> APDGKKGEAGR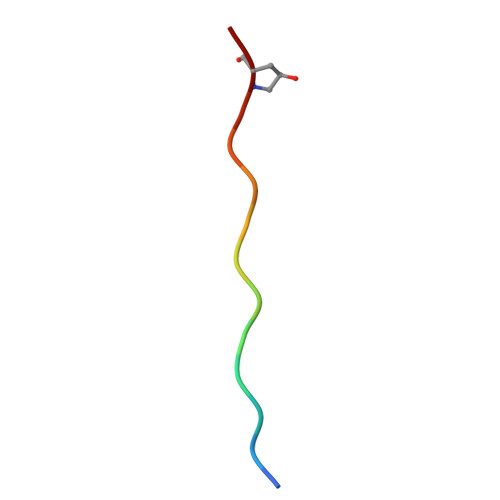PG> Q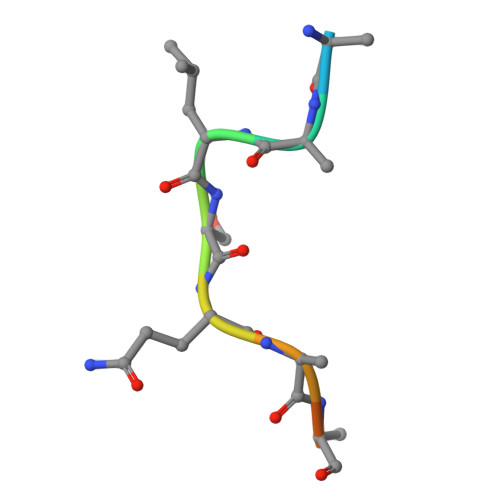PELSQDSYLG>MTSAEMTSPNNNSEHQAIAKMRTMIEGFDDISHGGLPIGRSTLVSGTSGTGKTLFSIQFLYNGIIEFDEPGVFVTFEETPQDIIKNARSFGWDLAKLVDEGKLFILDASPDPEGQEVVGGFDLSALIERINYAIQKYRARRVSIDSVTSVFQQYDASSVVRRELFRLVARLKQIGATTVMTTERIEEYGPIARYGVEEFVSDNVVILRNVLEGERRRRTLEILKLRGTSHMKGEYPFTITDHGINIFPLGAMRLTQRSSNVRVSSGVVRLDEMCGGGFFKDSIILATGATGTGKTLLVSRFVENACANKERAILFAYEESRAQLLRNAYSWGMDFEEMERQNLLKIVCAYPESAGLEDHLQIIKSEINDFKPARIAIDSLSALARGVSNNAFRQFVIGVTGYAKQEEITGLFTNTSDQFMGAHSITDSHISTITDTIILLQYVEIRGEMSRAINVFKMRGSWHDKAIREFMISDKGPDIKDSFRNFERIISGSPTRITVDEKSELSRIVRGVQEKGPES[6x];>[6x]MSPRKTYILKLYVAGNTPNSVRALKTLKNILEVEFQGVYALKVIDVLKNPQLAEEDKILATPTLAKVLPLPVRRIIGDLSDREKVLIGLDLLYGELQDSDDF;>MLSQIAICIWVESTAILQDCQRALSADRYQLQVCESGEMLLEYAQTHRDQIDCLILVAANPSFRAVVQQLCFEGVVVPAIVVGDRDSEDPDEPAKEQLYHSAELHLGIHQLEQLPYQVDAALAEFLRLAPVETMADHIMLMGANHDPELSSQQRDLAQRLQERLGYLGVYYKRDPDRFLRNLPAYESQKLHQAMQTSYREIVLSYFSPNSNLNQSIDNFVNMAFFADVPVTKVVEIHMELMDEFAKKLRVEGRSEDILLDYR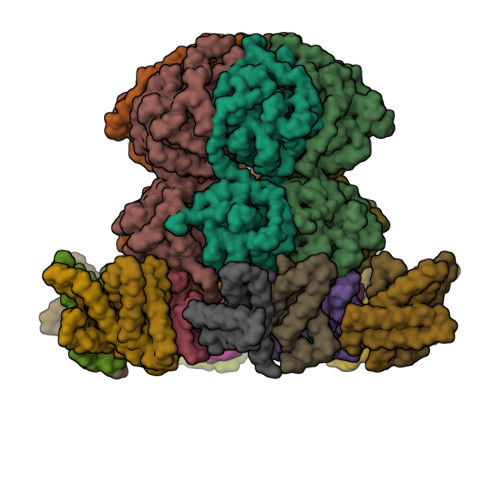LTLIDVIAHLCEMYRRSIPRET[12x]>MISVTLSQLTDILNGELQGADITLDAVTTDTRKLTPGCLFVALKGERFDAHDFADQAKAGGAGALLVSRPLDIDLPQLIVKDTRLAFGELAAWVRQQVPARVVALTGSSGKTSVKEMTAAILSQCGNTLYTAGNLNNDIGVPMTLLRLTPEYDYAVIELGANHQGEIAWTVSLTRPEAALVNNLAAAHLEGFGSLAGVAKAKGEIFSGLPENGIAIMNADNNDWLNWQSVIGSRKVWRFSPNAANSDFTATNIHVTSHGTEFTLQTPTGSVDVLLPLPGRH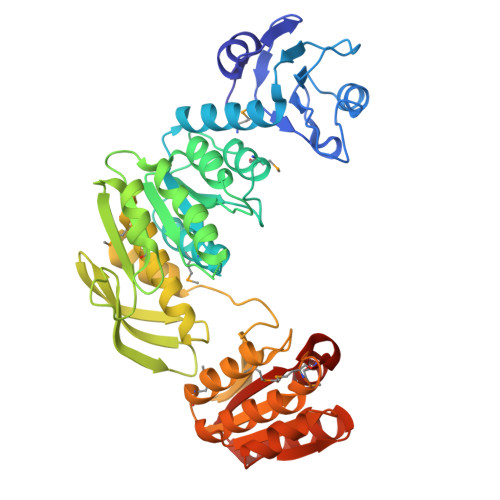NIANALAAAALSMSVGATLDAIKAGLANLKAVPGRLFPIQLAENQLLLDDSYNANVGSMTAAVQVLAEMPGYRVLVVGDMAELGAESEACHVQVGEAAKAAGIDRVLSVGKQSHAISTASGVGEHFADKTALITRLKLLIAEQQVITILVKGSRSAAMEEVVRALQENGTC[2x]>MASWSHPQFEKGADDDDKVPDPTSVDAVKHNRIKGIPKLDDANDAGGRNSTECTLILTEGDSAKTLAVSGLGVVGRDKYGVFPLRGKILNVREASHKQIMENAEINNIIKIVGLQYKKNYEDEDSLKTLRYGKIMIMTDQDQDGSHIKGLLINFIHHNWPSLLRHRFLEEFITPIVKVSKNKQEMAFYSLPEFEEWKSSTPNHKKWKVKYYKGLGTSTSKEAKEYFADMKRHRIQFKYSGPEDDAAISLAFSKKQIDDRKEWLTNFMEDRRQRKLLGLPEDYLYGQTTTYLTYNDFINKELILFSNSDNERSIPSMVDGLKPGQRKVLFTCFKRNDKREVKVAQLAGSVAEMSSYHHGEMSLMMTIINLAQNFVGSNNLNLLQPIGQFGTRLHGGKDSASPRYIFTMLSSLARLLFPPKDDHTLKFLYDDNQRVEPEWYIPIIPMVLINGAEGIGTGWSCKIPNFDVREIVNNIRRLMDGEEPLPMLPSYKNFKGTIEELAPNQYVISGEVAILNSTTIEISELPVRTWTQTYKEQVLEPMLNGTEKTPPLITDYREYHTDTTVKFVVKMTEEKLAEAERVGLHKVFKLQTSLTCNSMVLFDHVGCLKKYDTVLDILRDFFELRLKYYGLRKEWLLGMLGAESAKLNNQARFILEKIDGKIIIENKPKKELIKVLIQRGYDSDPVKAWKEAQQK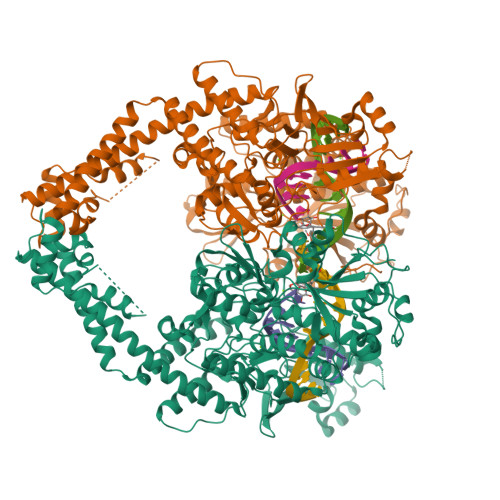VPDEEENEESDNEKETEKSDSVTDSGPTFNYLLDMPLWYLTKEKKDELCRLRNEKEQELDTLKRKSPSDLWKEDLATFIEELEAVEAKEKQDGAPGFSSISAHHHHHHHHHH[2x]> AERSELTIHPKEFTTFVRNFNPFLGATNLHTTTDFIYEPLVVFNEMHGNTPVFRLAENFQMSDDLMSVTFDIRKGVKWSDGEAFTADDVVYSFNLVKEKPELDQSGINSWVTGVEKVNDYQVKFRLSEANSNVPYEIAKVPVVPKHVWSKVKDPSTFTNENPVGSGPFTVIDTFTPQLYIQCENPNYWDAANLDVDCLRVPQIANNDQFLGKVVNGEMDWTSSFVPDIDRTYAAASPKHHYWYPPAGTQAFVVNFKNPDAAKNEALTNVDFRRAFSMALDRQTIIDIAFYGGGTVNDFASGLGYAFEAWSDEKTHDKFKAYNSYNAEGAKKLLAKAGFKDVNKDGFVDTPSGKSFELLIQSPNGWTDFNNTVQLAVEQLAEVGIKARARTPDFSVYNQAMLEGTYDVAYTNYFHGADPYTYWNSAYNSALQSGDGMPRAAMHFYKNEKLDGLLNSFYKTADKQEQLEIAHGIQQIIAQDQVTIPVLSGAYMYQYNTTRFTGWWNEENPKGRPNIWAGIPERLLHVLDLKPVKLEHHHHHH

VhCBP is a periplasmic chitooligosaccharide-binding protein mainly responsible for translocation of the chitooligosaccharide (GlcNAc)2 across the double membranes of marine bacteria. The chitooligosaccharide-specific SBP is localized to the periplasmic compartment of the bacterial cell wall and serves as a mobile component of the (GlcNAc)2-specific ABC transporter. SBPs share a common structural feature comprising two domains connected by a flexible hinge region. VcCBP and VhCBP belong to cluster C/subcluster IV (C-IV), members of which are specific for oligosaccharides, including mannooligosaccharides, cellooligosaccharides, and chitooligosaccharides.

A similar effect was observed in F437A, that is, the hydrophobic interaction with the N-acetyl methyl group of the reducing-end GlcNAc was likely eliminated by the F437A mutation; however, in this case, the hydrogen bonding network formed by the Arg436 side chain was partly affected by the Ala mutation of Phe437. F437A also showed a relatively large change in the binding affinity. By contrast, the reduction in hydrophobicity in the F437A mutation may not only have weakened hydrophobic interaction with the N-acetyl methyl group of the reducing-end GlcNAc at the site 2 but also added a conformational restraint to Phe411. The F437A mutation may have also affected the hydrogen bond network formed by the nearby amino acid, Arg436, with the N-acetyl carbonyl group of the same GlcNAc and with a bound water molecule. These subtle changes resulted in a rather large impact on ΔG° (ΔΔG° = +4.1 ± 0.3 kcal mol−1). The specificity toward GlcNAc may be mainly attributed to these two amino acids, indicating that mutational study of Arg436 and Phe437 may lead to specificity-engineered sugar-specific SBPs.> LVHVASVEKGRSYEDFQKVYNAIALKLREDDEYDNYIGYGPVLVRLAWHISGTWDKHD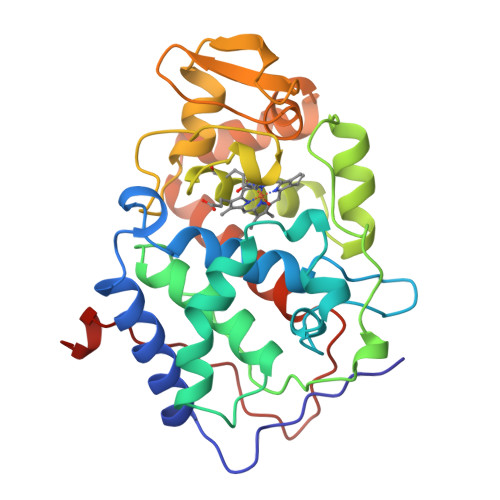NTGGSYGGTYRFKKEFNDPSNAGLQNGFKFLEPIHKEFPWISSGDLFSLGGVTAVQEMQGPKIPWRCGRVDTPEDTTPDNGRLPDADKDAGYVRTFFQRLNMNDREVVALMGAHALGKTHLKNSGYEGPGGAANNVFTNEFYLNLLNEDWKLEKNDANNEQWDSKSGYMMLPTDYSLIQDPKYLSIVKEYANDQDKFFKDFSKAFEKLLEDGITFPKDAPSPFIFKTLEEQGL> MNPPWAKPFELLVSFLNTPKYGTFDPTPVVPVFFPFWFGMIVGDIGYALLFYLVGRWLSGYVKRNEPLVIDLFALKLKPQVIGKLVHILNWMVFWTVVWGVIYGEFFGTFLEHLGVFGTPEHPGLIPILIHRIDTAKTANLLILLSVAFGVVLVFFGLALRAYLGLKHRHMAHFWEGVGYLGGLVGVLALAASYLGNLQAGWLQGLMYLGFGVFLLAVLMSRIWLMIPEIFTQAGHILSHIRIYAVGAAGGILAGLLTDVGFALAERLGLLGVLLGLLVAGVLHLLILLLTTLGHMLQPIRLL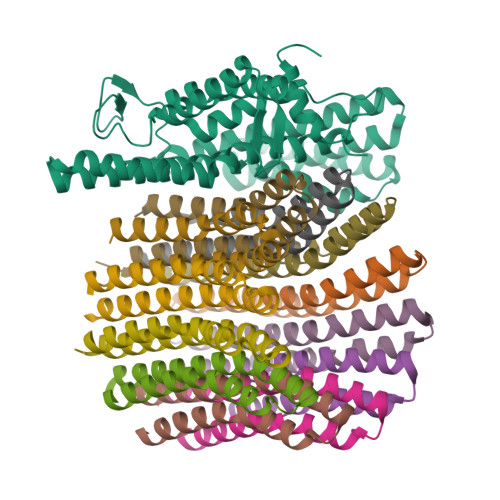WVEFFTKFGFYE;>SGGLDRGLIAVGMGLAVGLAALGTGVAQARIGAAGVGAIAEDRSNFGTALIFLLLPETLVIFGLLIAFILNGRL[12x]Specialized protein transport systems—known as type VII secretion systems (T7SSs)—are central to the virulence of this pathogen, and are also crucial for nutrient and metabolite transport across the mycobacterial cell envelope. Mycobacterium tuberculosis encodes five homologous, but functionally distinct, T7SSs that are designated ESX-1 to ESX-5. These systems translocate a number of effector proteins across the unique and impermeable diderm cell envelope. Here we reconstituted the ESX-5 T7SS of M. tuberculosis H37Rv in M. smegmatis to obtain a structural view of the entire T7SS membrane complex from this human pathogen.

At the cytoplasmic side of the complex, EccC5 has a stalk helix that connects its second TMH to the first NBD (which is also known as the DUF domain). This NBD is bound to the cytosolic domains of inner and outer EccD5, which—in turn—are bound to EccE5 at the periphery, together forming a ‘cytosolic bridge’. Further classification of the extended state reveals EccC5 to be more heterogenous beyond NBD1, which suggests that NBD1 is more stably bound to components of its own protomer. In the contracted state, the flexible arms of EccC5 extend from the interface between the DUF domain of EccC5 and the cytosolic domain of inner EccD5.

> MKRGFARPTPEKPPVIKPENIVLSTPLSIPPPEGKPWWLIVVGVVVVGLLGGMVAMVFASGSHVFGGIGSIFPLFMMVGIMMMMFRGMGGGQQQMSRPKLDAMRAQFMLMLDMLRETAQESADSMDANYRWFHPAPNTLAAAVGSPRMWERKPDGKDLNFGVVRVGVGMTRPEVTWGEPQNMPTDIELEPVTGKALQEFGRYQSVVYNLPKMVSLLVEPWYALVGEREQVLGLMRAIICQLAFSHGPDHVQMIVVSSDLDQWDWVKWLPHFGDSRRHDAAGNARMVYTSVREFAAEQAELFAGRGSFTPRHASSSAQTPTPHTVIIADVDDPQWEYVISAEGVDGVTFFDLTGSSMWTDIPERKLQFDKTGVIEALPRDRDTWMVIDDKAWFFALTDQVSIAEAEEFAQKLAQWRLAEAYEEIGQRVAHIGARDILSYYGIDDPGNIDFDSLWASRTDTMGRSRLRAPFGNRSDNGELLFLDMKSLDEGGDGPHGVMSGTTGSGKSTLVRTVIESLMLSHPPEELQFVLADLKGGSAVKPFAGVPHVSRIITDLEEDQALMERFLDALWGEIARRKAICDSAGVDDAKEYNSVRARMRARGQDMAPLPMLVVVIDEFYEWFRIMPTAVDVLDSIGRQGRAYWIHLMMASQTIESRAEKLMENMGYRLVLKARTAGAAQAAGVPNAVNLPAQAGLGYFRKSLEDIIRFQAEFLWRDYFQPGVSIDGEEAPALVHSIDYIRPQLFTNSFTPLEVSVGGPDIEPVVAQPNGEVLESDDIEGGEDEDEEGVRTPKVGTVIIDQLRKIKFEPYRLWQPPLTQPVAIDDLVNRFLGRPWHKEYGSACNLVFPIGIIDRPYKHDQPPWTVDTSGPGANVLILGAGGSGKTTALQTLICSAALTHTPQQVQFYCLAYSSTALTTVSRIPHVGEVAGPTDPYGVRRTVAELLALVRERKRSFLECGIASMEMFRRRKFGGEAGPVPDDGFGDVYLVIDNYRALAEENEVLIEQVNVIINQGPSFGVHVVVTADRESELRPPVRSGFGSRIELRLAAVEDAKLVRSRFAKDVPVKPGRGMVAVNYVRLDSDPQAGLHTLVARPALGSTPDNVFECDSVVAAVSRLTSAQAPPVRRLPARFGVEQVRELASRDTRQGVGAGGIAWAISELDLAPVYLNFAENSHLMVTGRRECGRTTTLATIMSEIGRLYAPGASSAPPPAPGRPSAQVWLVDPRRQLLTALGSDYVERFAYNLDGVVAMMGELAAALAGREPPPGLSAEELLSRSWWSGPEIFLIVDDIQQLPPGFDSPLHKAVPFVNRAADVGLHVIVTRTFGGWSSAGSDPMLRALHQANAPLLVMDADPDEGFIRGKMKGGPLPRGRGLLMAEDTGVFVQVAATEVRR;>[2x]MTAVADAPQADIEGVASPQAVVVGVMAGEGVQIGVLLDANAPVSVMTDPLLKVVNSRLRELGEAPLEATGRGRWALCLVDGAPLRATQSLTEQDVYDGDRLWIRFIADTERRSQVIEHISTAVASDLSKRFARIDPIVAVQVGASMVATGVVLATGVLGWWRWHHNTWLTTIYTAVIGVLVLAVAMLLLMRAKTDADRRVADIMLMSAIMPVTVAAAAAPPGPVGSPQAVLGFGVLTVAAALALRFTGRRLGIYTTIVIIGALTMLAALARMVAATSAVTLLSSLLLICVVAYHAAPALSRRLAGIRLPVFPSATSRWVFEARPDLPTTVVVSGGSAPVLEGPSSVRDVLLQAERARSFLSGLLTGLGVMVVVCMTSLCDPHTGQRWLPLILAGFTSGFLLLRGRSYVDRWQSITLAGTAVIIAAAVCVRYALELSSPLAVSIVAAILVLLPAAGMAAAAHVPHTIYSPLFRKFVEWIEYLCLMPIFPLALWLMNVYAAIRYR> AGSDPKCTEKEGNRTYNCENLGLREIPDTLPNTTEVLEFSFNFLPTIQNTTFSRLINLIFLDLTRCQINWVHEDTFQSHHQLNTIVLTGNPLIFMAETSLTGPKFLKHLFLTQTGISNLEFIPVHNLENLESLHLGS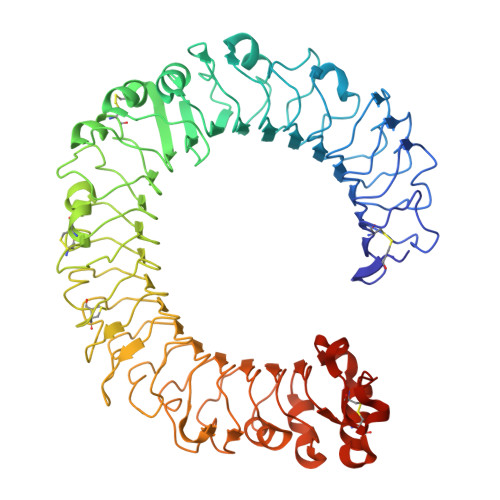NHISSINLPENFPTQNLKVLDFQNNAIHYISRKDTNSLEQATNLSLNFNGNDIKGIEPGAFISKIFQSLKFGGSLNLFIIFKGLQNSTLQSLWLGTFEDTDDQYLTSATFEGLCDMSVESINLQKHRFSDLSSSTFRCFTRVQELDLTAAHLNGLPSGIEGMNSLKKLVLNANSFDQLCQINAASFPSLRDLYIKGNMRKLDLGTRCLEKLENLQKLDLSHSDIEASDCCNLQLKNLRHLQYLNLSYNEPLGLEDQAFKECPQLELLDVAFTHLHVKAPHSPFQNLHLLRVLNLSHCLLDTSNQHLLAGLQDLRHLNLQGNSFQDGSISKTNLLQMVGSLEILILSSCNLLSIDQQAFHGLRNVNHLDLSHNSLTGDSMDALSHLKGLYLNMASNNIRIIPPHLLPALSQQSIINLSHNPLDCTCSNIHFITWYKENLHKLEDSEETTCANPPSLRGVKLSDVKLHCGTHMLVPR>[2x]GEFEKLEALEQLQSHIEGWEGSNLTDICTQLLLQGTLLKISAGNIQERAFFLFDNLLVYCKRKSRVTGSKKSTKRTKSINGSLYIF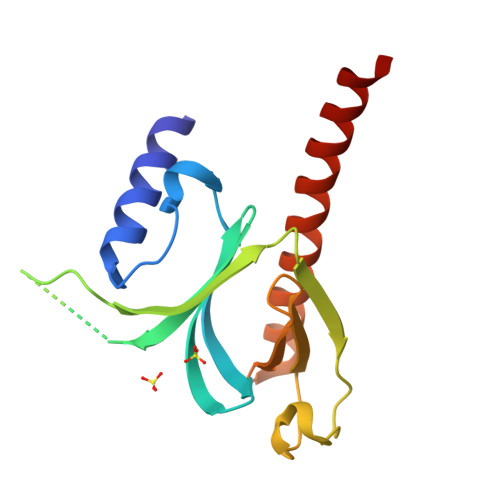RGRINTEVMEVENVEDGTADYHSNGYTVTNGWKIHNTAKNKWFVCMAKTAEEKQKWLDAIIREREQRESLKLGMERDAYVM>MGFAFKRGISTPDLALITRQLATLVQSGMPLEECLRAVAEQSEKP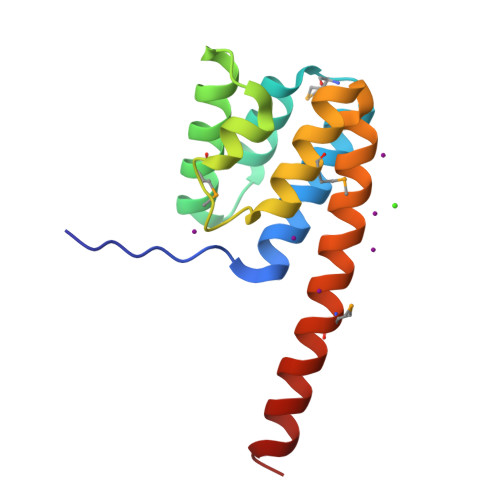RIRTMLVAVRAKVTEGYTLSDSLGDYPHVFDELFRSMVAAGEKSGHLDSVLERLADYAENRQKMRSKLQQASENLYPQ[2x]> PREVLTGGHSVSAPQENRIYVMDSVFMHLTESRVHVYDYTNGKFLGMVPTAFNGHVQVSNDGKKIYTMTTYHERITRGKRSDVVEVWDADKLTFEKEISLPPKRVQGLNYDGLFRQTTDGKFIVLQNASPATSIGIVDVAKGDYVEDVTAAAGCWSVIPQPNRPRSFMTICGDGGLLTINLGEDGKVASQSRSKQMFSVKDDPIFIAPALDKDKAHFVSYYGNVYSADFSGDEVKVDGPWSLLNDEDKAKNWVPGGYNLVGLH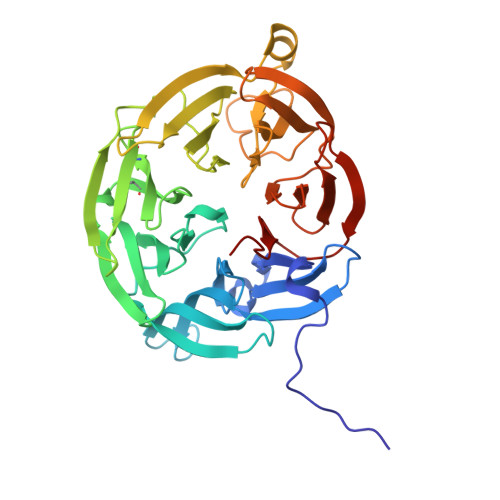RASGRMYVFMHPDGKEGTHKFPAAEIWVMDTKTKQRVARIPGRDALSMTIDQQRNLMLTLDGGNVNVYDISQPEPKLLRTIEGAAEASLQVQFHPVGGT1-beta-D-ribofuranosyl-1H-1,2,4-triazole-3-carboximidamide 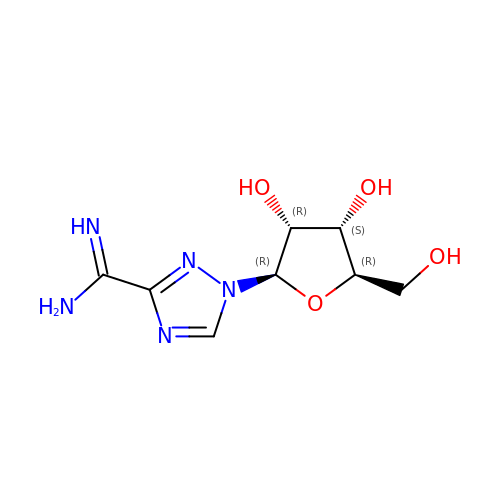| C8 H13 N5 O4 | NHKZSTHOYNWEEZ-AFCXAGJDSA-N>[2x]VAFGADAAKTTQEKFDALKEAGVFSGYPGTTDAKLGQDMTRAEFAKVLVKLFGLKEIHGQYSYKDKNYDAKNWAAPFIEAVTAEGLMQGKDLTKKIFDFNGKITVEEASKTLVTALKLEPVKDAQNKATDWAKGYFEAAVNAGLFSKDANPKANATRAQLVEAAFAADEMSKGSGSHHHHHH

Prokaryotic cell envelopes often include proteinaceous surface (S-) layers composed of self-assembling subunits in porous two-dimensional crystalline lattices. S-layer anchoring is best characterized for Gram-positive bacteria, where S-layer proteins non-covalently attach to the PG layer via species- and strain-specific non-classical secondary cell wall polymers (SCWPs). SpaA possesses three consecutive SLH domains near its N-terminus, followed by a large C-terminal region presumed to harbor the self-assembling domain(s). The crystal structures and binding analyses presented here of P. alvei SpaASLH, SpaASLH/G109A, and SpaASLH/G46A/G109A with synthetic SCWP fragments provide novel insights into the functional contributions of many conserved SLH domain residues, including SLH-Trp13, SLH-Gly29, and SLH-Arg43, which precisely interlock from three different SLH domains to generate two active binding sites.

Here we report crystal structures of the SLH domains of SpaA, unliganded and in complex with synthesized monosaccharide and disaccharide building blocks of P. alvei CCM 2051T SCWP. The TRAE, TVEE, and TRAQ motifs of SpaA are located at the N-termini of the core helices adjacent to three grooves (labeled here G1, G2, and G3). The TRAE and TRAQ motifs each contribute to two of the three grooves, as their arginine residues thread under the connecting loops of the adjacent SLH domains and into the neighboring grooves. In the case of SLH2, Val125 of the TVEE motif corresponds in position to the conserved SLH-Arg43 of the TRAE and TRAQ motifs but does not protrude into the neighboring G3. In the initial liganded and unliganded structures, multiple conformations were observed for residues 44–54 that form the connecting loop between the two helices of SLH1 beside G1. The loop makes unique crystal contacts in each case and has mean B-factors elevated between 4 and 49% of the molecule mean. In both G1 and G2, the non-conserved SLH-28 residue is observed to make a hydrogen bond from its backbone carbonyl to the side chain of the conserved SLH-Arg43 of the TRAE motif. The hydrogen bond between the SLH-28 backbone carbonyl and SLH-Arg43 in the unliganded state may support the proper folding of the SLH domain trimer, as these residues precisely interlock between neighboring SLH domains.>GMPSEKQPQSKGNKMAILKLDEHLYISPQLTKADAEQIAQLGIKTIICNRPDREEESQPDFAQIKQWLEQAGVTGFHHQP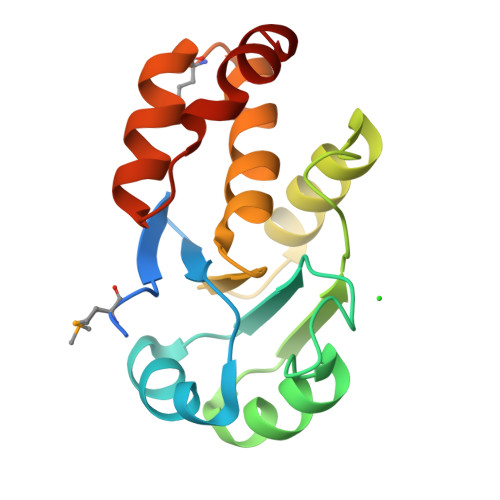VTARDIQKHDVETFRQLIGQAEYPVLAYCRTGTRCSLLWGFRRAAEGMPVDEIIRRAQAAGVNLENFRERLDNARV[2x]>MDSKQQRIGVIGTGAIGGFYGLMLAHAGHDVHFLLRSEFEAVNRAGLSLNSAVHGFRRLAPVQAYHSAQDMPPCDWLLVGAKTTGNHELAPLIRAAAAPGAKVLLLQNGLGVEERLRPLLPESLHLLGGLCFICVHRGEPGVIEHQAYGGVNLGYHSGPADERRRREIVEEGAALFRESGLESTAMPDLEQARWQKLVWNIPYNGLSVLLKSSTAPLMANADSRSLIEAIMEEVIGAAGACGFILPEGYADQLLAATERMPDYRPSMYHDFAHGRPLELAAIYAAPLAR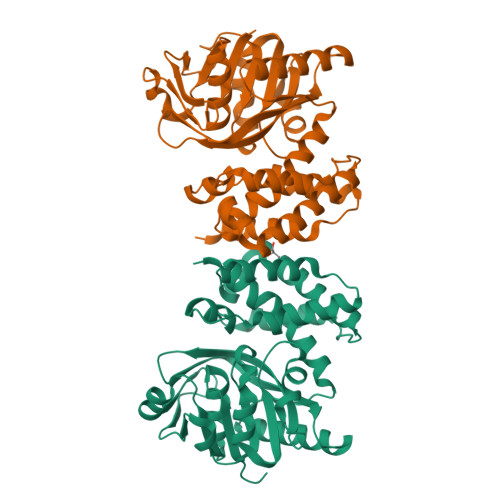AAAAGYRMPRVEALHQALRFLEAQPR[2x]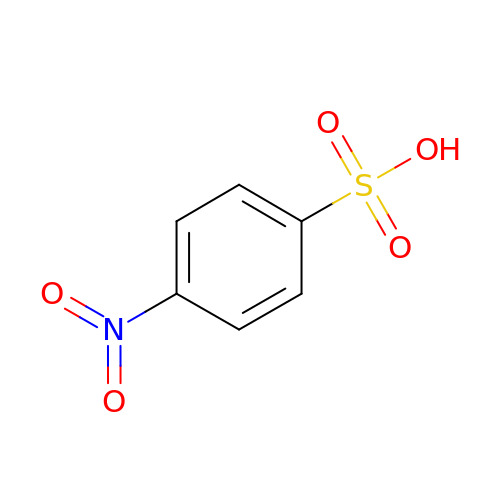4-nitrobenzenesulfonic acid | C6 H5 N O5 S | SPXOTSHWBDUUMT-UHFFFAOYSA-N>NKRAPYWTNTEKMEKRLHAVPAANTVKFRCPAGGNPMPTMRWLKNGKEFKQEHRIGGYKVRNQHWSLIMESVVPSDKGNYTCVVENEYGSINHTYHLDVV[2x];>NYKKPKLLYCSNGGHFLRILPDGTVDGTRDRSDQHIQLQLSAESVGEVYIKSTETGQYLAMDTD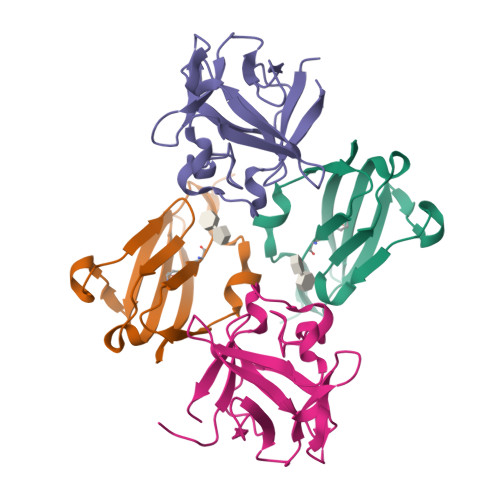GLLYGSQTPNEECLFLERLEENHYNTYISKKHAEKNWFVGLKKNGSCKRGPRTHYGQKAILFLPLPV[2x]> GAMVLTQTHATGHVGDFFFTHWKDGGSTSLTLDAEGKFLVTWQGGGYNYVGGPGWHFGDKNRVIRYKLNEETGASYIALYGWGYDKTMSESDPSHLVEYYILQRWTYDPSQDGIYGKTFVSNGIEYSTYRSIRKVKPSINGPTTFYQYWSKPSAQQELGKDHKIIFADHVKAWADTGW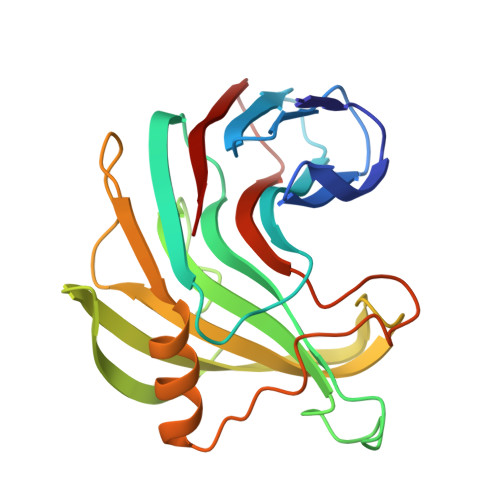ILPDMNNFDASDDPTYQVLAVEVFNPQKNGTASGQVWDE> MEGVYTVTVYPGDPAFEIQDSLPQKIWPMLYLHQQRWLPSYGPWHIRFTSSAMQLRNFPRSLRGQANFQNSMSLKLITALTDVISRISLDFYSDLRHLSDTMSALCLIAAYYSEKNQTPLPTNLPELLGNITAKVTLLVRDLKRAAANKGFNFNRNSSSLLPAQGGLYSNDFFQEHALYSLFRTAGMLASSSSPEYPRADSVLAITAAVFGDNIPPFAAYQWNLRSGLKALESLILLFLLLDVNVPATSNKRLHLEALLGESYSKGSRPPARRTGPLDAGGSVFSFLMENYLVPTLLHRPTTNMSALFPGLYLLQLEFSSGASTPHAIHLTDVKFRDIFNILVQSNVFQDSQELIRAKQSLRVSCETGSGNLLESLSPGTTMRDIIRKEFMAQDVYDYVYFCVLGALPVTVAVVPAAALEHHHHHHHHH

Herpesviruses cause severe diseases particularly in immunocompromised patients. Both genome packaging and release from the capsid require a unique portal channel occupying one of the 12 capsid vertices. Recent symmetry-relaxed cryo-EM reconstruction strategies of α- and γ-herpesviral virions provided first snapshots of the unique portal vertex that is essential for DNA encapsidation and release. These studies revealed for the first time a pentameric cap on top of the portal that presumably seals the capsids against DNA leakage after packaging and has been proposed to consist of pUL25 in HSV-1 and its ortholog pORF19 in KSHV. Here, we report the crystal structures of the CTDs of pUL25 orthologs from 3 members of the β- and γ-herpesviruses (HCMV, KSHV, and murid gammaherpesvirus 68 (MuHV-68)), highlighting their structural conservation across the herpesvirus subfamilies. The overall structures of the HSV-1, HCMV, KSHV, and MuHV-68 orthologs are well conserved as reflected by high z scores resulting from structural comparisons using the Dali server and in spite of a low amino acid identity within the “twilight zone” (approximately 20% between the crystallized fragments of HSV-1 pUL25 and MuHV-68 pORF19; illustrated in the structural alignment in S3 Fig).

Similar to HSV-1 pUL25CTD, pUL77CTD and pORF19MCTD crystallized as a monomer. Pentameric portal caps have been demonstrated in α- and γ-herpesviruses; however, neither HSV-1 pUL25CTD nor MuHV-68 pORF19MCTD are pentameric in solution or in the crystal, suggesting that additional triggers or stabilizing forces are required for pentamerization. The crystal structure of the HSV-1 pUL25 CTD displays a remarkable charge distribution with a number of positively charged residues on one face of the molecule (blue in S4A Fig) and a cluster of negatively charged residues on the opposite face. A similar but more pronounced polarization in the electrostatic potential was observed in pUL77CTD, whereas the corresponding surfaces of the γ-herpesviral orthologs did not reveal any accumulation of charged residues. (E) View on the MuHV-68 pORF19 CTD (pORF19MCTD) shown in surface representation with residues conserved across all 4 orthologs colored in yellow. A larger conserved patch consisting of 4 residues distant in primary sequence (colored in orange) is in close proximity to the loop connecting Y365 and S384 (black arrows), which is disordered in the crystal structures of all orthologs, suggesting that the conserved patch is likely buried in the native protein.>[2x]MCGIFAYLNYHVPRTRREILETLIKGLQRLEYRGYDSAGVGFDGGNDKDWEANACKIQLIKKKGKVKALDEEVHKQQDMDLDIEFDVHLGIAHTRWATHGEPSPVNSHPQRSDKNNEFIVIHNGIITNYKDLKKFLESKGYDFESETDTETIAKLVKYMYDNRESQDTSFTTLVERVIQQLEGAFALVFKSVHFPGQAVGTRRGSPLLIGVRSEHKLSTDHIPILYRTGKDKKGSCNLSRVDSTTCLFPVEEKAVEYYFASDASAVIEHTNRVIFLEDDDVAAVVDGRLSIHRIKRTAGHHHHHHDHPGRAVQTLQMELQQIMKGNFSSFMQKEIFEQPESVVNTMRGRVNFDDYTVNLGGLKDHIKEIQRCRRLILIACGTSYHAGVATRQVLEELTELPVMVELASDFLDRNTPVFRDDVCFFLSQSGETADTLMGLRYCKERGALTVGITNTVESSISRETDCGVHINAGPEIGVASTKAYTSQFVSLVMFALMMCDDRISMQERRKEIMLGLKRLPDLIKEVLSMDDEIQKLATELYHQKSVLIMGRGYHYATCLEGALKIKEITYMHSEGILAGELKHGPLALVDKLMPVIMIIMRDHTYAKCQNALQQVVARQGRPVVICDKEDTETIKNTKRTIKVPHSVDCLQGILSVIPLQLLAFHLAVLRGYDVDFPRNLAKSVTVE

In the first step of the HP, GFAT synthesizes d-glucosamine-6-phosphate (GlcN6P) from l-glutamine (l-Gln) and Frc6P, releasing l-glutamate (l-Glu). GFAT contains two domains: the glutaminase domain responsible for releasing ammonia in the hydrolysis of l-Gln to l-Glu and the isomerase/transferase domain, which catalyzes both the isomerization of Frc6P to d-glucose-6-phosphate (Glc6P) as well as the transfer of ammonia to Glc6P to produce GlcN6P. The active sites of the two domains are linked by an ammonia channel, which forms when GFAT engages with both of its substrates, l-Gln and Frc6P. The main distinctive feature between prokaryotic and eukaryotic GFAT is the feedback inhibition by the HP product UDP-GlcNAc, which inhibits the glutaminase function.

Having solved the structure of GFAT-1, we aimed to understand the mechanism of GFAT-1 activation through a single amino acid substitution (G451E) that elevated HP flux and extended lifespan in C. elegans. Positioned in an evolutionary conserved region of the isomerase domain, Gly451 is in close proximity to the UDP-GlcNAc-binding site, suggesting that the mutation might interfere with UDP-GlcNAc inhibition. Crystal structure analysis of GFAT-1 G451E revealed no major structural changes compared to wild type GFAT-1. Notably, Glu451 forms a new hydrogen bond to Gln307 of the interdomain linker in the mutant structure. Analysis of the kinetic properties of the G451E mutant revealed a comparable Km for l-Gln-hydrolysis but had a reduced kcat compared to the wild type enzyme. Very remarkably, however, GFAT-1 G451E showed a drastically reduced sensitivity to UDP-GlcNAc feedback inhibition. We conclude that GFAT-1 gain-of-function in the G451E variant results from a loss of regulation by UDP-GlcNAc-mediated feedback inhibition. In our mutants, we observed altered sensitivities to UDP-GlcNAc, which we interpret as follows: in the gain-of-function mutant G451E, which showed a reduced sensitivity to UDP-GlcNAc inhibition, the hydrogen bond between Glu451 and Gln307 stabilizes the linker and both residues might function as spacers between the interdomain linker and the UDP-GlcNAc-bound isomerase domain, preventing a close interaction.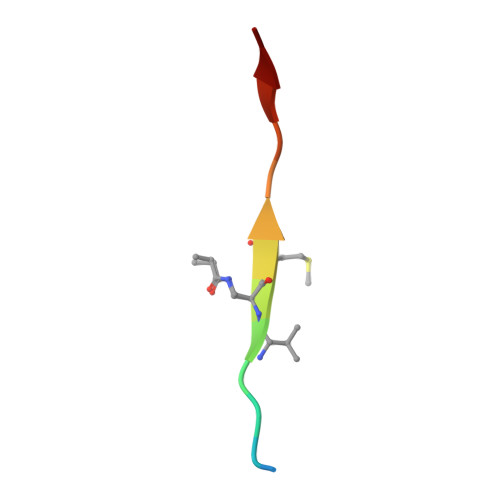> XKLRPVXMVRPWVR>DQGGEEEEDYESEEQLQHRILTAALEFVPAHGWTAEAIAEGAQSLGLSSAAASMFGKDGSELILHFVTQCNTRLTRVLEEEQKLVQLGQAEKRKTDQFLRDAVETRLRMLIPYIEHWPRALSILMLPHNIPSSLSLLTSMVDDMWHYAGDQSTDFNWYTRRAMLAAIYNTTELVMMQDSSPDFEDTWRFLENRVNDAMNM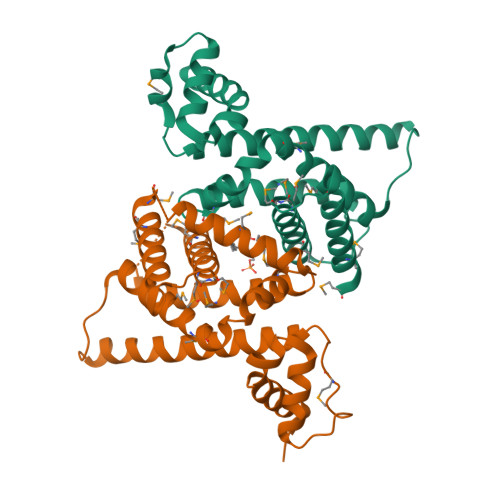GHTAKQVKSTGEALVQGLMGAAVTLKNLTGLNQRR[2x]> LENKPRIPVVWIHGLECTCCTESFIRSAHPLAKDVILSLISLDYDDTLMAAAGTQAEEVFEDIITQYNGKYILAVEGNPPLGEQGMFCISSGRPFIEKLKRAAAGASAIIAWGTCASWGCVQAARPNPTQATPIDKVITDKPIIKVPGCPPIPDVMSAIITYMVTFDRLPDVDRMGRPLMFYGQRIHDKCYRRAHFDAGEFVQSWDDDAARKGYCLYKMGCKGPTTYNACSSTRWNDGVSFPIQSGHGCL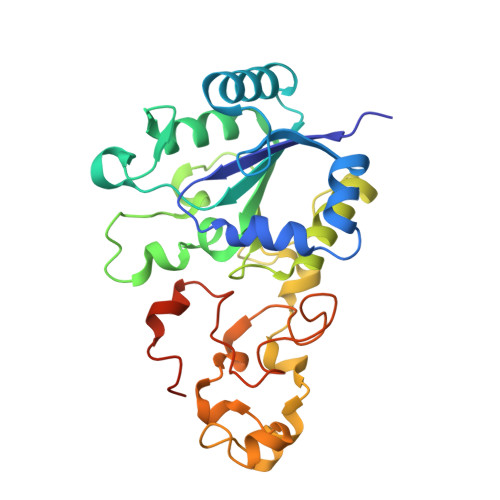GCAENGFWDRGSFYSRGSFYSRHHHHHH> GSMLISHSDMNQQLKSAGIGFNATELHGFLSGLLCGGLKDQSWLPLLYQFSNDNHAYPTGLVQPVTELYEQISQ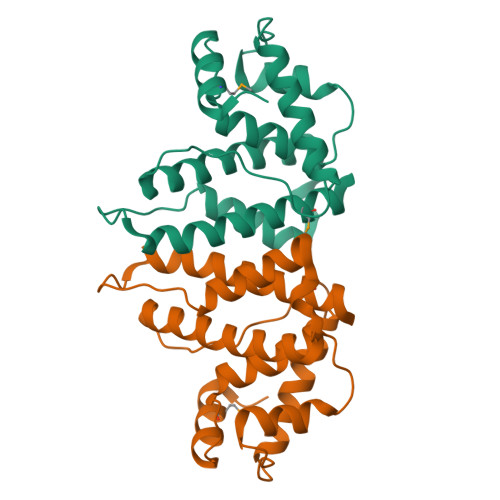TLSDVEGFTFELGLTEDENVFTQADSLSDWANQFLLGIGLAQPELAKEKGEIGEAVDDLQDICQLGYDEDDNEEELAEALEEIIEYVRTIAMLFYSHFNEGEIESKPVLH5-(2-CHLOROPHENYL)FURAN-2-CARBOXYLIC ACID | C11 H7 Cl O3 | 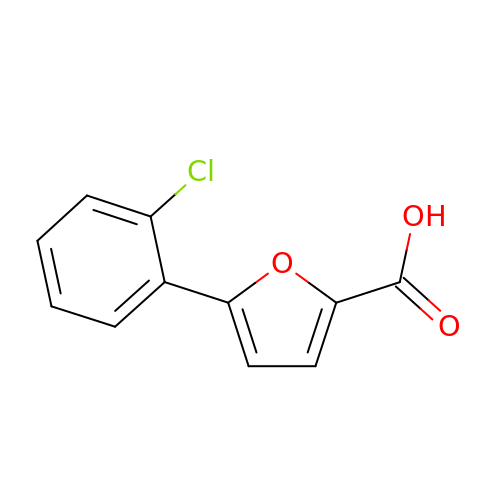PJGGWIHXGHQXMM-UHFFFAOYSA-N> QNSQFQSLEQVKRRPAHLMALLQHVALQFEPGPLLCCLHADMLGSLGPKEAKKAFLDFYHSFLEKTAVLRVPVPPNVAFELDRTRADLISEDVQRRFVQEVVQSQQVAVGRQLEDFRSKRLMGMTPWEQELAQLEAWVGRDRASYEARERHVAERLLMHLEEMQHTISTDEEKSAAVVNAIGLY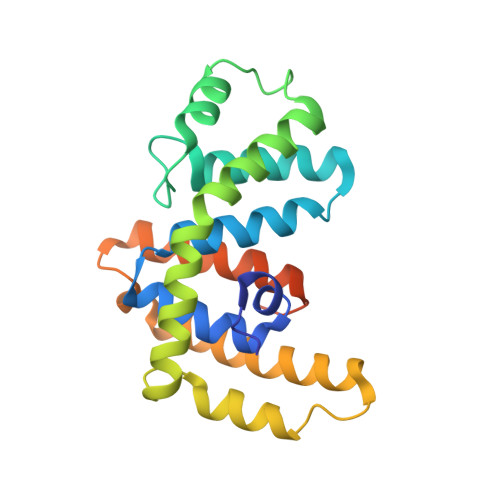MRHLGVRTKSGDKKSGRNFFRKKVMGN> LETPGQYLVYNGDLVEYEADHMAQLQRVHGFLMNDCLLVATWLPQRRGMYRYNALYPLDRLAVVNVKDNPPMKDMFKLLMFPESRIFQAENAKIKREWLEVL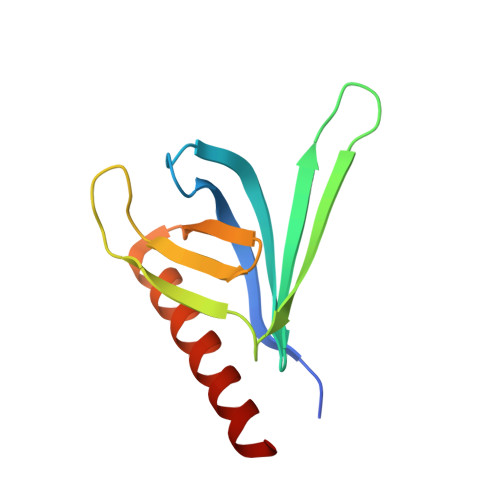EETKRALSDKR> SMQGPRTRPRKPIRCGEVLFAVGGWCSGDAISSVERYDPQTNEWRMVASMSKRRCGVGVSVLDDLLYA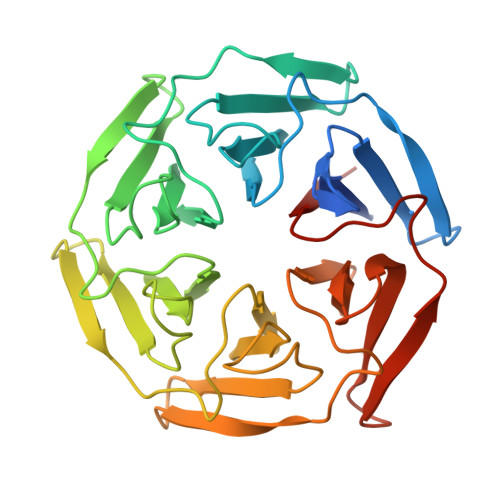VGGHDGSSYLNSVERYDPKTNQWSSDVAPTSTCRTSVGVAVLGGFLYAVGGQDGVSCLNIVERYDPKENKWTRVASMSTRRLGVAVAVLGGFLYAVGGSDGTSPLNTVERYNPQENRWHTIAPMGTRRKHLGCAVYQDMIYAVGGRDDTTELSSAERYNPRTNQWSPVVAMTSRRSGVGLAVVNGQLMAVGGFDGTTYLKTIEVFDPDANTWRLYGGMNYRRLGGGVGVIKMTHCE4-(5-{[(3-aminophenyl)methyl]carbamoyl}thiophen-2-yl)-1-benzothiophene-2-carboxamide | C21 H17 N3 O2 S2 | 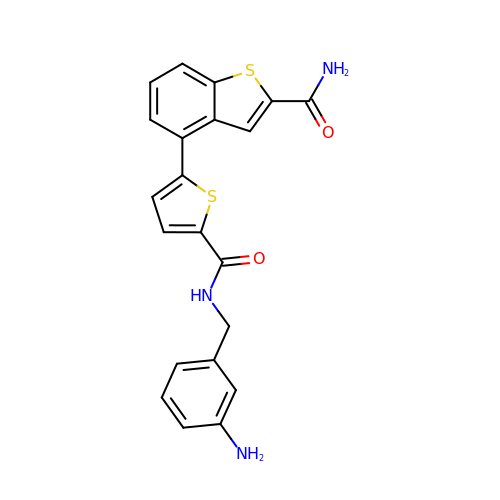SDZHQRUPXPKDOD-UHFFFAOYSA-N>[10x]MHHHHHHMPQTNPFHSLVPR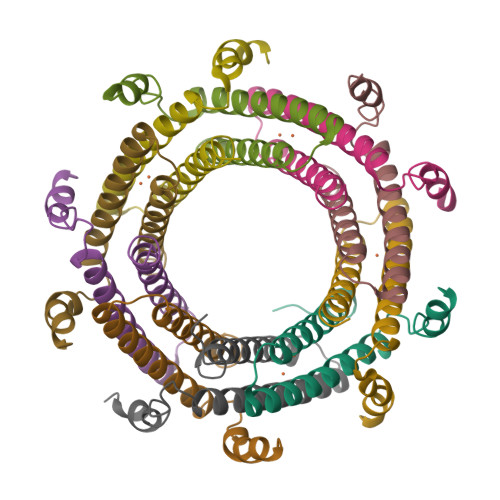KMTDTELARSIRLNIEAELDAINLYAAHIDATDNEDAKAILQHVMDEEREHAALFWELIARLDPEQAAHAKEAVEKYRLITSGASHEAVEAVGKEGAAPSPADVTPEKRLTVGSLRR RNRs produce all four deoxyribonucleotides and are the only enzymes providing de novo building blocks for DNA replication and repair in all free-living organisms. Class III RNRs, which only function anaerobically, are dimers of an α subunit (NrdD) with a stable radical close to the active site, and binding sites for allosteric nucleotides. Binding of ATP activates RNR, and binding of dATP inhibits it. Here, we present structural, biochemical, and biophysical studies on the ATP-cone-containing NrdD from the human pathogen Prevotella copri (PcNrdD; Nii et al., 2023), showing that the binding of dATP causes increased flexibility of the C-terminal glycyl radical-bearing domain, as well as a flap-like loop that binds across the top of the active site in the active form.

To investigate whether substrate had any allosteric effect on the conformations of the ATP-cone, flap, and GRD, we determined separate cryo-EM structures of tetrameric and dimeric PcNrdD, from the same grid, in the presence of 0.5 mM dATP and 0.5 mM CTP, achieving a resolution of 2.6 Å from 1,105,348 particles before post-processing for the tetramer and 2.6 Å from 1,132,695 particles for the dimer. Both forms were almost identical to those seen in the presence of dATP alone, and no CTP could be seen bound to the active site. In both forms, the C-terminal GRD is highly mobile in all monomers such that it cannot be seen in the cryo-EM reconstructions. Furthermore, the GRD is mobile in all complexes with dATP in the a-site, whether dimeric or tetrameric. Since both the ATP-cone and the GRD are disordered in the dATP-bound dimers, the exact molecular mechanism by which dATP induces disorder of the GRD remains somewhat elusive.

>[2x]GPGSMIQTVVKRDGRIVGFNEQKIMAAIRKAMLHTDKGEDTTLIEQITDHISYRGKSQMSVEAIQDAIEMELMKSARKDVAQKYIAYRNQRNIARKAKTRDVFMSIVNAKNNDITRENANMNADTPAGMMMKFASETTKPFVDDYLLSEDVRDAVMHNYIHIHDKDYYPTKSLTCVQHPLDVILNHGFTAGHGSSRPAKRIETAAVLACISLETCQNEMHGGQAIPAFDFYLAPYVRMSYQEEVKNLEKLTGEDLSNLYDAPIDDYIEKPLDGLQGRERLEQHAINKTVNRVHQAMEAFIHNMNTIHSRGGNQVVFSSINYGTDTSAEGRCIMREILQSTYQGVGNGETAIFPIQIWKKKRGVNYLPEDRNYDLYKLACKVTARRFFPNFLNLDATFNQNEKWRADDPERYKWEIATMGCRTRVFEDRWGEKTSIARGNLSFSTINIVKLAIECMGIENEKQRIDMFFAKLDNILDITAKQLDERFQFQKTAMAKQFPLLMKYLWVGAENLKPEETIESVINHGTLGIGFIGLAECLVALIGKHHGESEKAQELGLKIITYMRDRANEFSEQYHHNYSILATPAEGLSGKFTKKDRKQFGVIPGVTDRDYYTNSNHVPVYYKCTALKKAQIEAPYHDLTRGGHIFYVEIDGDATHNPSVIESVVDMMDKYNMGYGSVNHNRNRCLDCGYENADAHLEVCPKCGSHHIDKLQRITGYLVGTTDRWNSGKLAELHDRVTHIGGEK Voltage-gated sodium (Nav) channels are part of membrane-embedded signaling complexes that initiate the rising phase of action potentials, a crucial event in generating and propagating electrical signals throughout the human body. As key components of these protein assemblies, β-subunits (1) modify Nav channel-gating properties; (2) regulate channel trafficking and localization to distinct surface compartments; and (3) influence channel oligomerization. Structurally, β-subunits are single-transmembrane segment glycoproteins with a short cytoplasmic C-terminal tail and a large V-type immunoglobulin (Ig) extracellular domain that may participate in homophilic and heterophilic interactions, cell adhesion, and cell migration. Of the four known β-subunits and their splice variants (β1–4; gene names Scn1b-Scn4b), β2 and β4 form a disulfide bond with an unidentified Cys within particular Nav channel isoforms.

In addition to 55Cys, the hβ2 crystal structure reveals a unique motif bearing a protruding disulfide-stabilized loop formed by 72Cys and 75Cys. To determine if this loop regulates the gating or pharmacological influence of hβ2 on hNav1.2, we mutated 72Cys and 75Cys to Ala (C72A C75A) but found that it is functionally indistinguishable from WT hβ2. The lack of effect of the C72A C75A mutant on hNav1.2 function suggests that this disulfide bond is not essential for folding, and that its disruption may not significantly affect the position or environment of 55Cys. To verify this hypothesis, we produced recombinant hβ2 extracellular domain containing three Cys mutations: C55A, C72A, and C75A. Size exclusion chromatography demonstrates that the mutant produces monomeric protein, indicating that the bond between 72Cys and 75Cys is unessential for folding. Furthermore, we obtained a crystal structure of the triple mutant at 1.85Å which overlays well onto the C55A structure. The only significant difference is situated in the loop containing both cysteines, which now displays a single conformation. Although the spatial organization of this loop does not seem to impact the ability of hβ2 to modulate hNav1.2 gating or sensitivity to ProTx-II, this region may yet play a functional role in modulating other Nav channel isoforms.

>SNAMEVTVPATLNVLNGSDARLPCTFNSAYTVNHKQFSLNWTYQEANNASEEMFLQFRMKIINLKLERFQDRVEFSGNPSKYDVSVMLRNVQPEDEGIYNCYIMNPPDRHRGHGKIHLQVLMEEPPE[2x]>[4x]SNAMSGNVGAGRHADELAIRTVQYRWLEATRKFDRQVLSSLMTDDVVFLTPGRLPFGKEEFLAACEQNDQRVIIEASATFEEIVIVEPMAYTR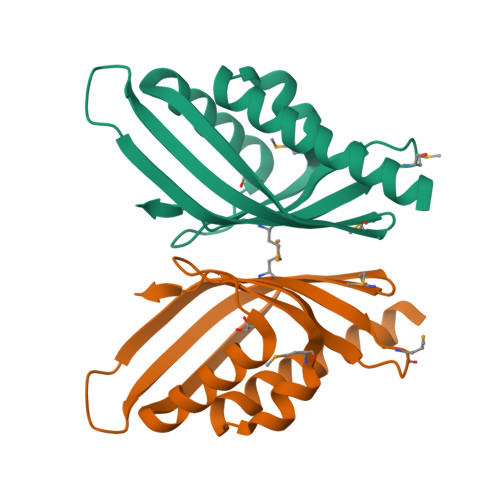THLHIKVTPRSGGAVRELAGHAMSIFRRSMFGEWQLARDANLVVPI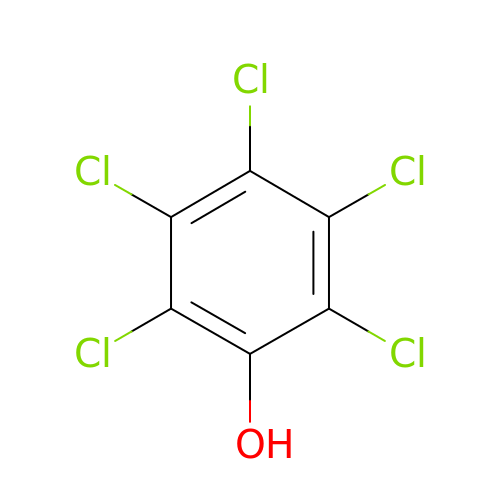PENTACHLOROPHENOL | C6 H Cl5 O | IZUPBVBPLAPZRR-UHFFFAOYSA-N> MKLMIVGNTGSGKTTLLQQLMKTKKSDLGMQSATVGIDVKDWPIQIRDKRKRDLVLNVWDFAGREEFYSTHPHFMTQRALYLAVYDLSKGQAEVDAMKPWLFNIKARASSSPVILVGTHLDVSDEKQRKACMSKITKELLNKRGFPAIRDYHFVNATEES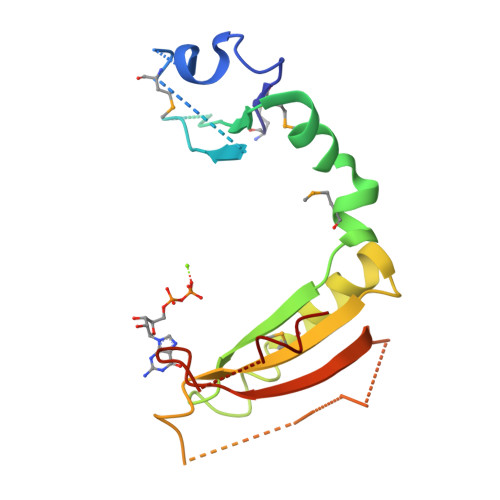DALAKLRKTII>[16x]VLPENMKRYMGRDAQRMNILAGRIIAETVRSTLGPKGMDKMLVDDLGDVVVTNDGVTILREMSVEHPAAKMLIEVAKTQEKEVGDGTTTAVVVAGELLRKAEELLDQNVHPTIVVKGYQAAAQKAQELLKTIACEVGAQDKEILTKIAMTSITGKGAEKAKEKLAEIIVEAVSAVVDDEGKVDKDLIKIEKKSGASIDDTELIKGVLVDKERVSAQMPKKVTDAKIALLNCAIEIKETETDAEIRITDPAKLMEFIEQEEKMLK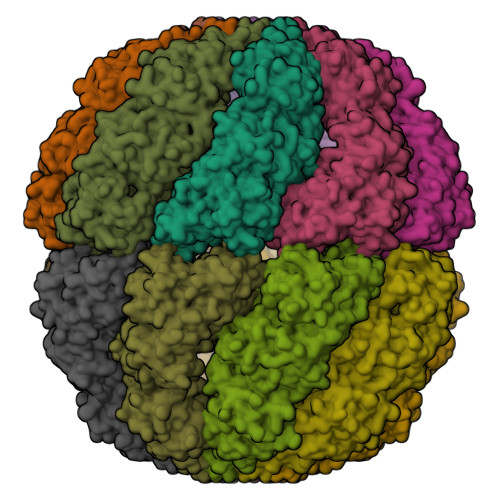DMVAEIKASGANVLFCQKGIDDLAQHYLAKEGIVAARRVKKSDMEKLAKATGANVIAAIAALSAQDLGDAGLVEERKISGDSMIFVEECKHPKAVTMLIRGTTEHVIEEVARAVDDAVGVVGCTIEDGRIVSGGGSTEVELSMKLREYAEGISGREQLAVRAFADALEVIPRTLAENAGLDAIEILVKVRAAHASNGNKCAGLNVFTGAVEDMCENGVVEPLRVKTQAIQSAAESTEMLLRIDDVIAAE>MHHHHHHEPLILTAAITGAETTRADQPNLPITPEEQAKEAKACFEAGARVIHLHIR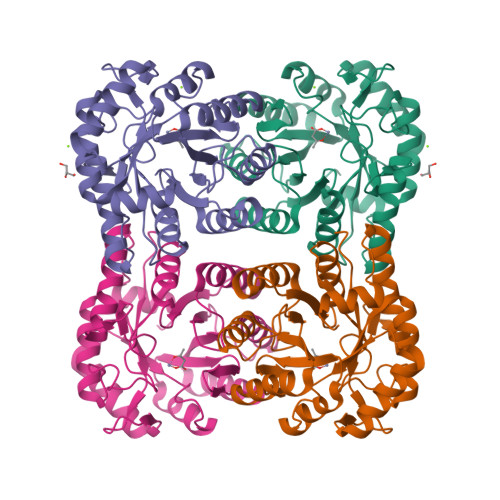EDDGRPSQRLDRFQEAISAIREVVPEIIIQISTGGAVGESFDKRLAPLALKPEMATLNAGTLNFGDDIFINHPADIIRLAEAFKQYNVVPEVEVYESGMVDAVARLIKKGIITQNPLHIQFVLGVPGGMSGKPKNLMYMMEHLKEEIPTATWAVAGIGRWHIPTSLIAMVTGGHIRCGFEDNIFYHKGVIAESNAQLVARLARIAKEIGRPLATPEQAREILALNK[2x]>GSVHKHTGRNCGRKFKIGEPLYRCHECGCDDTCVLCIHCFNPKDHV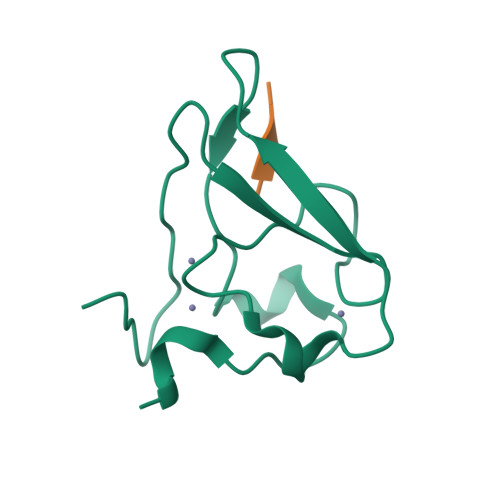NHHVCTDICTEFTSGICDCGDEEAWNSPLHCKAEEQ[2x];>[2x]RLGES> MRRNIFCLACLWIVQACLSLDRADILYNIRQTSRPDVIPTQ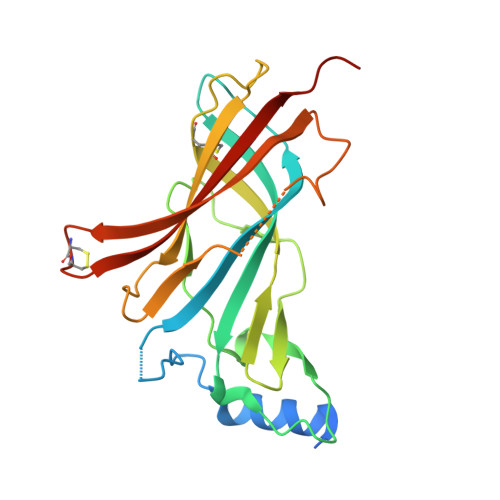RDRPVAVSVSLKFINILEVNEITNEVDVVFWQQTTWSDRTLAWNSSHSPDQVSVPISSLWVPDLAAYNAISKPEVLTPQLAHVVSDGEVQYTPSIRQRFSCDVSGVDTESGATCRIKIGSWTHHSREISVDPTTENSDDSEYFSQYSRFEILDVTQKKNSVTYSCCPEAYEDVEVSLNFRKKGRSEIL>MSGKRALITGIRGQDGAYLAKLLLEKGYEVYGADRRSGEFASWRLKELGIENDVKIIHMDLLEFSNIIRTIEKVQPDEVYNLAAQSFVGVSFEQPILTAEVDAIGVLRILEALRTVKPDTKFYQASTSEMFGKVQEIPQTEKTPFYPRSPYAVAKLFGHWITVNYREAYNMFACSGILFNHESPLRGIEFVTRKITYSLARIKYGLQDKLVLGNLNAKRDWGYAPEYVEAMWLMMQQPEPDDYVIATGETHTVREFVEKAAKIAGFDIEWVGEGINEKGIDRNTGKVIVEVSEEFFRPAEVDILV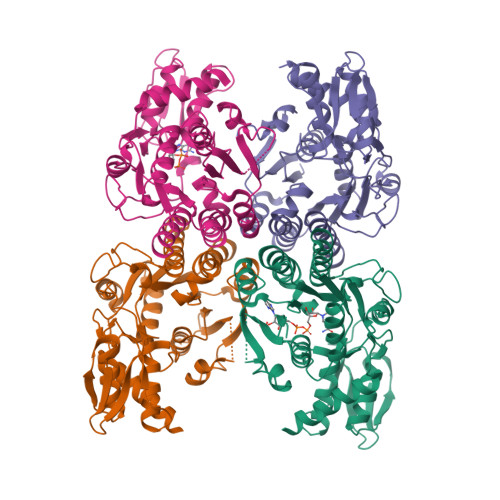GNPEKAMKKLGWKPRTTFDELVEIMMEADLKRVRDREVSV[4x]>MYYSNGNYEAFADPKKPAGVDKKSAYIIGSGLAGLSTAVFLVRDAQMKGENIHILEELPVAGGSLDGADRPNAGFVVRGGREMENHFECLWDMYRSIPSLEVPGASYLDEYYWLDKEDPNSSNCRLIYNRGDRLPSDGQYGLGKCANEIVKLIMTPEKEIEGQTIEEFFSDEFFKTNFWTYWSTMFAFEKWHSLAEMRRYAMRFIHHIDGLPDFTALKFNKYNQYESMVKPLLAYLKDHGVQFEYDCHVKNVEVDHEGDSKIAKKIVMTQNGKDKEIDLTHNDIVFVTNGSITESSTYGDQNTPAPITNAKGDSWKLWENLAKQDPAFGHPDVFCENLPERSWFVSATATLENKKLAPYFERLTKR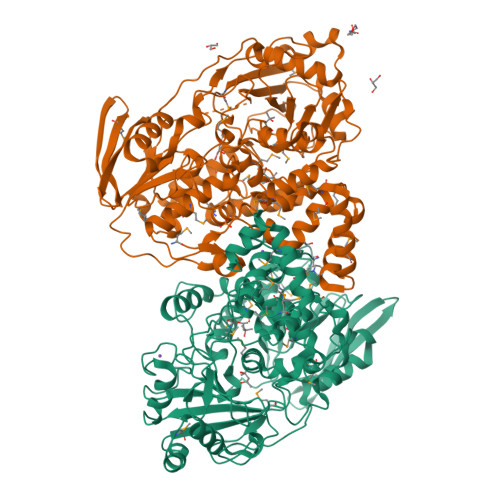SLYDGKVNTGGIITIVDSNWELSFTIHRQPHFKSQNPDQIVVWIYALYSDTEGNYIKKRIVDCTGKEIAEELLYHLGVPESQISELASEENMNTVPVYMPYITSYFMPRRDGDRPDVVPEGSINLAFIGNFAESPTRDTVFTTEYSVRTAMEAVYTLLNVDRGVPEVFDSIYDIRQLLRAMYYMSDKKKLADQDMPLPEKLAVKTGMRKIKKTWVEELLKEANLV[2x]> MGKKSRVKTQKSGTGATATVSPKEILNLTSELLQKCSSPAPGPGKEWEEYVQIRTLVEKIRKKQKGLSVTFDGKREDYFPDLMKWASENGASVEGFEMVNFKEEGFGLRATRDIKAEELFLWVPRKLLMTVESAKNSVLGPLYSQDRILQAMGNIALAFHLLCERASPNSFWQPYIQTLPSEYDTPLYFEEDEVRYLQSTQAIHDVFSQYKNTARQYAYFYKVIQTHPHANKLPLKDSFTYEDYRWAVSSVMTRQNQIPTEDGSRVTLALIPLWDMCNHTNGLITTGYNLEDDRCECVALQDFRAGEQIYIFYGTRSNAEFVIHSGFFFDNNSHDRVKIKLGVSKSDRLYAMKAEVLARAGIPTSSVFALHFTEPPISAQLLAFLRVFCMTEEELKEHLLGDSAIDRIFTLGNSEFPVSWDNEVKLWTFLEDRASLLLKTYKTTIEEDKSVLKNHDLSVRAKMAIKLRLGEKEILEKAVKSAAVNREYYRQQMEEKAPLPKYEESNLGLLESSVGDSRLPLVLRNLEEEAGVQDALNIREAISKAKATENGLVNGENSIPNGTRSENESLNQESKRAVEDAKGSSSDSTAGVKE;> GKFGQQSGAIYVGNFRVVNRHLATHNDWANLVWEDSSRDLLVSSTTAQGCDTIARCNCQTGVYYCNSRRKHYPVSFSKPSLIYVEASEYYPARYQSHLMLAQGHSEPGDAGGILRCQHGVVGIVSTGGNGLVGFADVRDLLWLDEEAMEQ

SETD3 is an essential host factor for the replication of a variety of enteroviruses that specifically interacts with viral protease 2A. SETD3 functions as an actin-specific histidine N-methyltransferase, and comprises an N-terminal SET domain and a C-terminal Rubisco large subunit methyltransferase (LSMT) like domain. The N- and C-terminal domains of SETD3 form a V-shaped central cleft, within which the actin substrate is recognized and methylated at residue H7318,19.

Specifically, SETD3 1−503 coexpressed with EV71 2A in insect cells was suitable for cryo-electron microscopy (EM) studies, and separately produced SETD3 1−498 and EV71 2A from E. coli were suitable for in vitro complex assembly and crystallization. The poor resolution of our X-ray diffraction data motivated us to switch to a single-particle cryo-EM approach for structural investigation. The coexpressed SETD3 1−503-EV71 2A complex from sf21 cells was suitable for sample vitrification and data collection. Although the molecular mass of this complex was only 73 kDa, we obtained a 3.1 Å cryo-EM density map providing further structural details. We could locate residues 21−501 of SETD3 and residues 6−146 of EV71 2A in the EM density (Supplementary Fig. 3&4). There are two discrete contacts between SETD3 and EV71 2A domain II, denoted Site-1 and Site-2. Comparing the two independently determined SETD3-2A complex structures showed that while the conformation of each component was highly similar (RMSD between the crystal and EM structures of EV71 2A was 0.49 Å, and that between SETD3 structures was 0.64 Å), their relative positions were slightly shifted, which contributes to the increased overall RMSD to 1.20 Å. We then aligned the crystal and EM structures with respect to SETD3, and identified a rotation between SETD3 and 2A. The rotational axis runs along the β-bII1 strand of EV71 2A, where 2A engages in an intermolecular antiparallel β-strand interaction with the SETD3 SET domain through two backbone hydrogen bonds. Structural variation between the crystal and EM structures reflects a degree of flexibility in the SETD3-2A interaction.> MESLPVIAAPSMWTRPQIRDFKEKIRQDSDSVITVGRGEVVTVRVPTHEEGSYLFWEFATDNYDIGFGVYFEWTD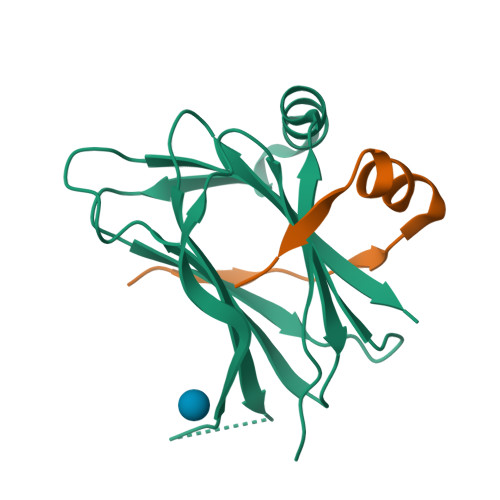SPNTAVSVHVSESSEHDDEEEEENISSEEKAKKNANKPVLDEIVPVYRRDCHEEVYAGSHQYPGRGVYLLKFDNSYSLWRSKSVYYRVYYTR;> GLTIEAEPTELSYQDALEMLAESKPVSTTLSFER> MKTWPAPTAPTPVRATVTVPGSKSQTNRALV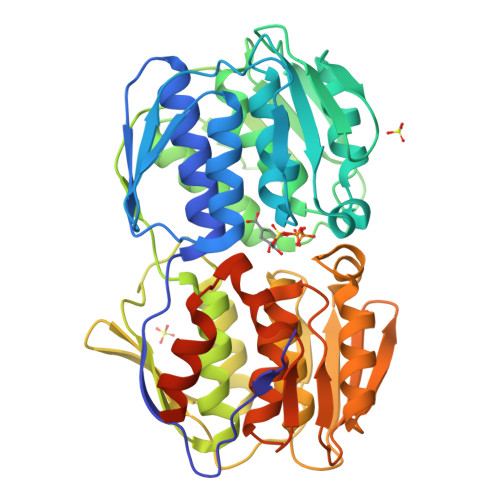LAALAAAQGRGASTISGALRSRDTELMLDALQTLGLRVDGVGSELTVSGRIEPGPGARVDCGLAGTVLRFVPPLAALGSVPVTFDGDQQARGRPIAPLLDALRELGVAVDGTGLPFRVRGNGSLAGGTVAIDASASSQFVSGLLLSAASFTDGLTVQHTGSSLPSAPHIAMTAAMLRQAGVDIDDSTPNRWQVRPGPVAARRWDIEPDLTNAVAFLSAAVVSGGTVRITGWPRVSVQPADHILAILRQLNAVVIHADSSLEVRGPTGYDGFDVDLRAVGELTPSVAALAALASPGSVSRLSGIAHLRGHETDRLAALSTEINRLGGTCRETPDGLVITATPLRPGIWRAYADHRMAMAGAIIGLRVAGVEVDDIAATTKTLPEFPRLWAEMVGPGQGWGYPQPRSGQRARRATGQGSGG>HHHHHHENLYFQGSGSSPRSGVLLRGCPTHCHCEPDGRMLLRVDCSDLGLSELPSNLSVFTSYLDLSMNNISQLLPNPLPSLRFLEELRLAGNALTYIPKGAFTGLYSLKVLMLQNNQLRHVPTEALQNLRSLQSLRLDANHISYVPPSCFSGLHSLRHLWLDDNALTEIPVQAFRSLSALQAMTLALNKIHHIPDYAFGNLSSLVVLHLHNNRIHSLGKKCFDGLHSLETLDLNYNNLDEFPTAIRTLSNLKELGFHSNNIRSIPEKAFVGNPSLITIHFYDNPIQFVGRSAFQHLPELRTLTLNGASQI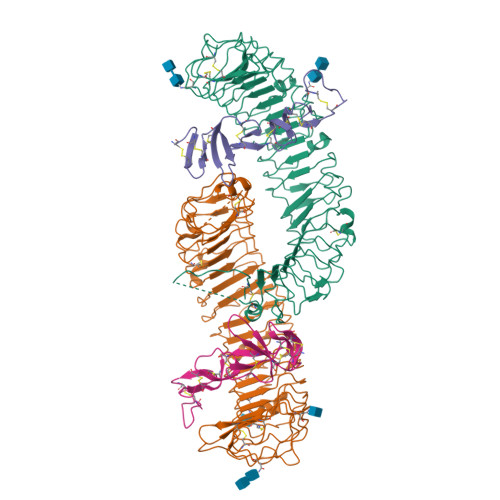TEFPDLTGTANLESLTLTGAQISSLPQTVCNQLPNLQVLDLSYNLLEDLPSFSVCQKLQKIDLRHNEIYEIKVDTFQQLLSLRSLNLAWNKIAIIHPNAFSTLPSLIKLDLSSNLLSSFPITGLHGLTHLKLTGNHALQSLISSENFPELKVIEMPYAYQCCAFGVCENAYKISNQWNKGDNSSMDDLHKKDAGMFQAQDERDLEDFLLDFEEDLKALHSVQCSPAAA[4x];>[4x]GSRISAEGSQACAKGCELCSEVNGCLKCSPKLFILLERNDIRQVGVCLPSCPPGYFDARNPDMNKCIKCKIEHCEACFSHNFCTKCKEGLYLHKGRCYPACPEGSSAANGTMECSSPAAAHHHHHH>[2x]MHPGFFTSIGQMTDLIHTEKDLVTSLKDYIKAEEDKLEQIKKWAEKLDRLTSTATKDPEGFVGHPVNAFKLMKRLNTEWSELENLVLKDMSDGFISNLTIQRQYFPNDEDQVGAAKALLRLQDTYNLDTDTISKGNLPGVKHKSFLTAEDCFELGKVAYTEADYYHTELWMEQALRQLDEGEISTIDKVSVLDYLSYAVYQQ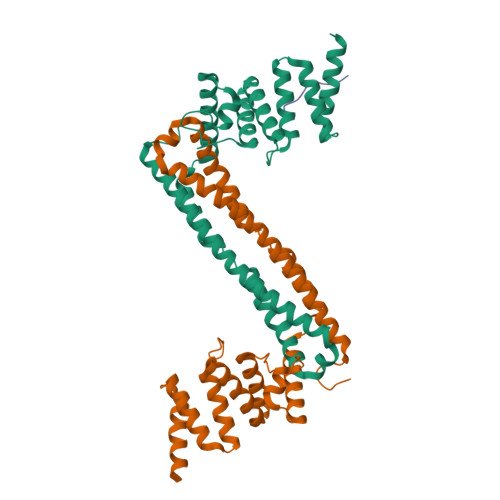GDLDKALLLTKKLLELDPEHQRANGNLKYFEYIMAKE;> PPGPPGPPG>[4x]MGHHHHHHSGENLYFQGASMRTLLIRYILWRNDGDPSYYNDDFKKLILFDELVDDDDVCTLIKNMRMTLSDGPLLDRLNQPVNNVEDVKRMIAISAKVARDIG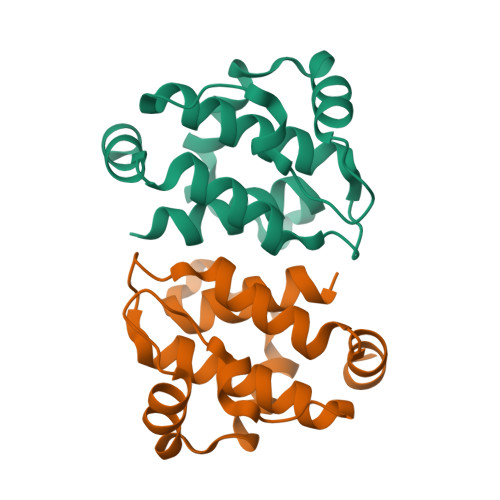RRPEIRWEDSFTILFRMIEKYFDDLMTDLYGEK>[2x]SGAFEDRDPTQF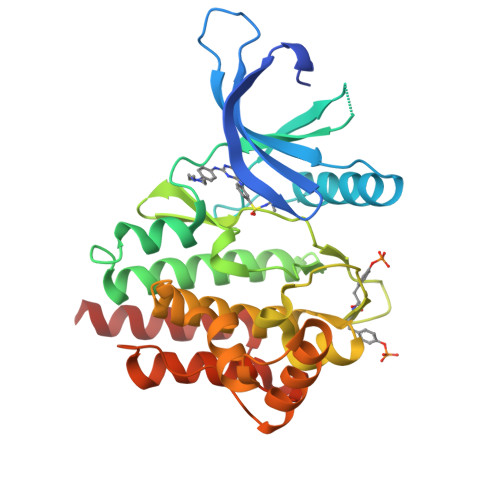EERHLKFLQQLGKGNFGSVEMCRYDPLQDNTGEVVAVKKLQHSTEEHLRDFEREIEILKSLQHDNIVKYKGVCYSAGRRNLKLIMEYLPYGSLRDYLQKHKERIDHIKLLQYTSQICKGMEYLGTKRYIHRDLATRNILVENENRVKIGDFGLTKVLPQDKEYYKVKEPGESPIFWYAPESLTESKFSVASDVWSFGVVLYELFTYIEKSKSPPAEFMRMIGNDKQGQMIVFHLIELLKNNGRLPRPDGCPDEIYMIMTECWNNNVNQRPSFRDLALRVDQIRDNMAG> MSADLQQGTTNAADFSLTVLRARIALLATAIGGPDYTSQIDPPPYKLGDDCLACLKDLKRWFKLVDDQQKRWDVAMAVAEYRILTDDLLPILIDWENKCSLAAKLAKNNPD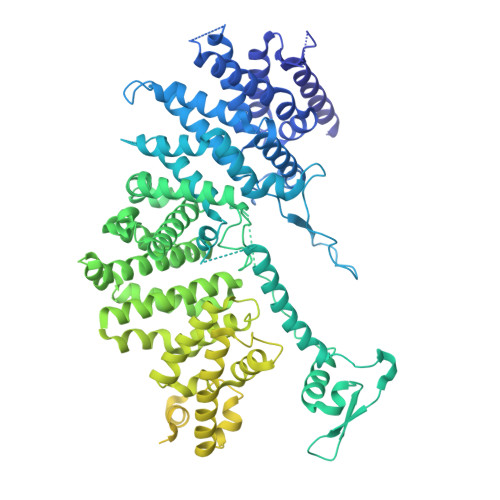HEEFRNKAYYDKIALNCLQLLVLMTWPLIVTEQSSSNQITLYGELKKHQLVYKKTILSMESGKVLRAAIRLALDVIKIDRLSRTPRDNMVLKLVLNFFRNVIAIEPGEFTINTKKSMPKKGITSIDTLPPNVSMDDISLNTVISSFHKNKVFGFLLTLTSSLSKEFDQDFINIPLLEIMFYFTKDVNQELLFPRQFETGTHSKVVNKNESSSANNIVTSAGFELSKLLQKEHQMRKNVIKHTSARHSRFGGLLSIQTPDKTRLTVSGSQALVDEKIALQKLDDSKKWNKRIIKKHQSVAAEGLPNSLLNSQTGKAIFFTESNGKHFKEFINNFIDSGFNILLHSVTNYFTTEQDRMVTLEQVEYLLFFAWFVKYQLLRSKIDNSADIKQVSEALKEVTFILVSSLLRSAYDLKNWTVTHAGMIAFNELLNLVSRTKAAQEEDSTDIEFIVSRLFSDERIQLLSNLPKIGSKYSLQFMKSCIELTHSVLKVLEQYSDDKTLVIEGKSRRQKKFNISEGDITKLIEEENVDRDEALDILTSSLRSIEVNFQKVQANYMTEPVIETYINFLERFRELEDDSIKKVFSFFHRVFVQAKEQALLFRFDLIILLREMLSPDGLDRMSRSRKYVSQFSDYFLARLKKRLKKSPAWFVGLLFPPLHNSEVGFYQRYGEYNVLNNESMYAAPASQFKPIPDEEALPPSILLDMKYGVLVSTLLDDGKTELLDQLLKHITHTLDIFKSWLTVNVNAGKETVNPPNEYFTLTGVLNNDPIFKDKDYRALLLLIGYSIPRKINEPCFLPGTVEVSDLTVSCELVKKYLSTPFETPNGLPSSSYLLRVRSEKDSFSHNEQDGWEGDDDYDYNDPYIVPDDQILSKSDAAYFKDLDNNASDKLKGTKFSKGIARSKKKDKRKRRKGEAKTNLPMFGDQDDERPQTVRERHGVFSKEFISDSEDDEDLMNPIFFENETYMRWLLDKNNGQLTEDRYIQFAKFAAERMNNGGVVTGDYTSLFGGSIPSIESIRATESSSFAPDKSLISLASHVASEMSIFDVNNNNNNQLSDDDVNSESRNSLGSSQPSNSQNMFQSEVYSRKESTKRSLEASAADESDEDEEAIRLFGKKSRVVLSQGDSDD> MRGSHHHHHHGSSKKTTTVGVIIPDISSIFYSELARGIEDIATMYKYNIILSNSDQNMEKELHLLNTMLGKQVDGIVFMGGNITDEHVAEFKRSPVPIVLAASVEEQEETPSVAIDYEQAIYDAVKLLVDKGHTDIAFVSGPMAEPINRSKKLQGYKRALEEANLPFNEQFVAEGDYTYDSGLEALQHLMSLDKKPTAILSATDEMA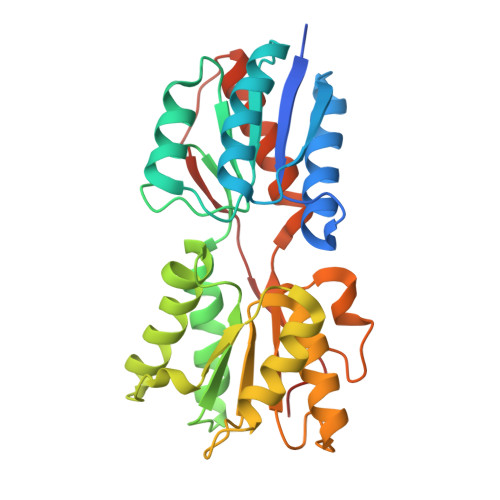LGIIHAAQDQGLSIPEDLDIIGFDNTRLSLMVRPQLSTVVQPTYDIGAVAMRLLTKLMNKEPVEEHIVELPHRIELRKSTKS> SNAMKIAAFDIGGTALKMGVVLPHGEIILTKSAEISGSDGDQILAEMKVFLAENTDVTGIAVSAPGYVNPKTGLITMGGAIRRFDNFNLKEWLEAETGLPVAIENDANCALLAEKWLGKGQDLDDFLCLTIGTGIGGGIFSNGELVRGGRFRAGEFGYMFSERPGAFRPGKYTLNETTTMLVLRRQYAELTGRPLEEITGEEIFANYDAHDAVSERLITEFYTG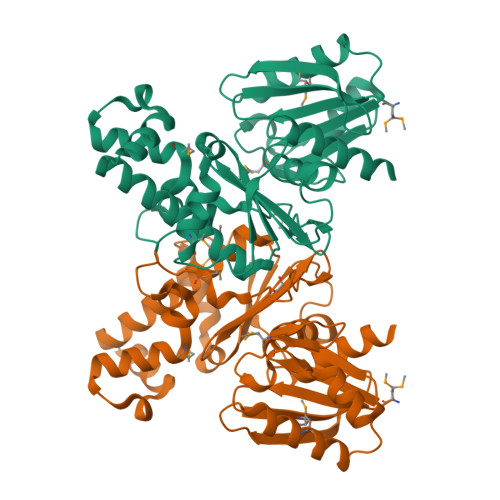ICTGLYNLIYLFDPTHIFIGGGITSRPTFIAELKHHMESFGLRDTIIETATHKNQAGLLGAVYHFLQEENRHE> AFGITTSSSAYVIDTNAPNQLKFTVSRSSCDITSIIHYGTELQYSSQGSHIGSGLGSATVTATQSGDYIKVTCVTDTLTQYMVVHNGDPIIHMATYITAEPSIGELRFIARLNSDLLPNEEPFGDVSTTADGTAIEGSDVFLVGSETRSKFYSSERFIDDQRHCIAGDAHRVCMILNQYESSSGGPFHRDINSNNGGSYNALYWYMNSGHVQTESYRMGLHGPYSMYFSRSGTPSTSIDTSFFADLDIKGYVAASGRGKVAGTASGADSSMDWVVHWYNDAAQYWTYTSSSGSFTSPAMKPGTYTMVYYQGEYAVATSSVTVSAGSTTTKNISGSVKTGTTIFKIGEWDGQPTGFRNAANQLRMHPSDSRMSSWGPLTYTVGSSALTDFPMAVFKSVNNPVTIKFTATSAQTGAATLRIGTTLSFAGGRPQATINSYTGSAPAAPTNLDSRGV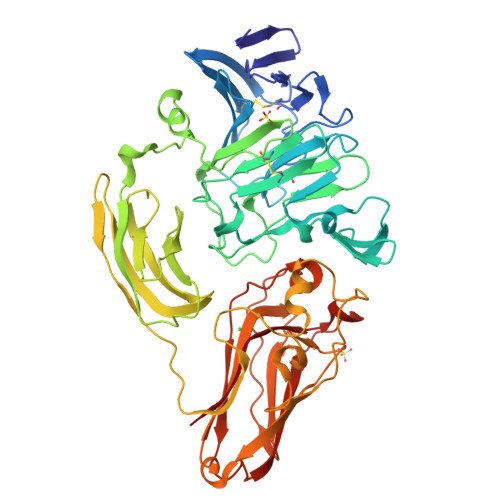TRGAYRGLGEVYDVSIPSGTIVAGTNTITINVISGSSGDTYLSPNFIFDCVELFQ> MGHMPERFDAFICYCPSDIQFVQEMIRQLEQTNYRLKLCVSDRDVLPGTCVWSIASELIEKRCRRMVVVVSDDYLQSKECDFQTKFA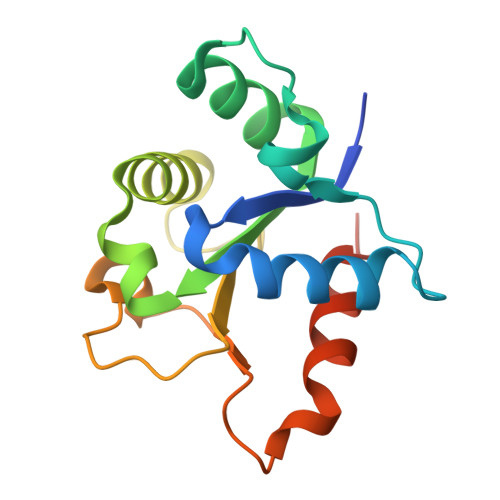LSLSPGAHQKRLIPIKYKAMKKEFPSILRFITVCDYTNPCTKSWFWTRLAKALSLPLEHHHHHH>MEVEKEFITDEAKELLSKDKLIQQAYNEVKTSICSPIWPATSKTFTINNTEKNCNGVVPIKELCYTLLEDTYNWYREKPLDILKLEKKKGGPIDVYKEFIENSELKRVGMEFETGNISSAHRSMNKLL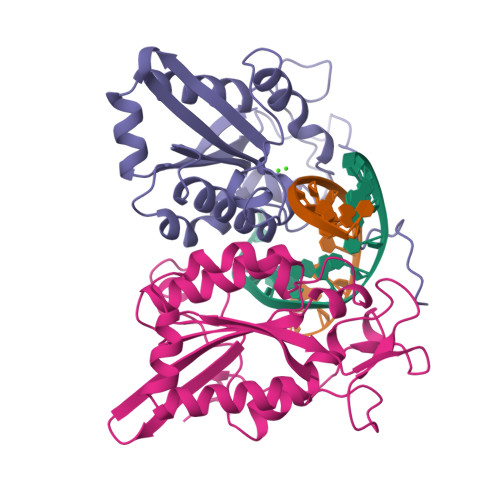LGLKHGEIDLAIILMPIKQLAYYLTDRVTNFEELEPYFELTEGQPFIFIGFNAEAYNSNVPLIPKGSDGMSKRSIKKWKDKVENK[2x]> MKVDLNADAGESYGAFAYGHDREIFPLVSSANLACGFHGGSPGRILEAVRLAKAHGVAVGAHPGFPDLVGFGRREMALSPEEVYADVLYQIGALSAFLKAEGLPLHHVKPHGALYLKACRDRETARAIALAVKAFDPGLPLVVLPGTVYEEEARKAGLRVVLEAFPERAYLRSGQLAPRSMPGSWITDPEEAARRALRMVLEGK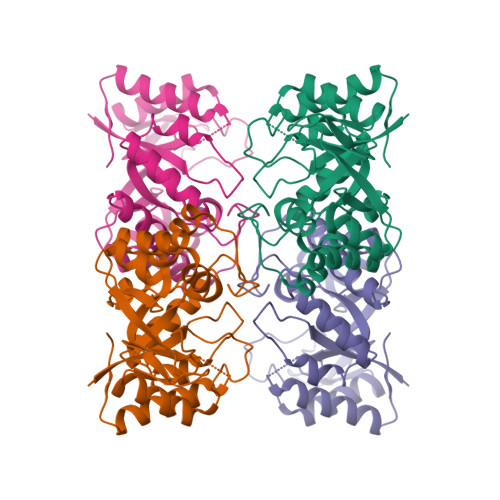VEALDGGEVAVRADTLCIHGDNPNAPEVARAVREALEQAGVEVRAF> MGSSHHHHHHSSGENLYFQGHMSNTSWRKSEVLAVPLQPTLQQEVILARMEQILASRALTDDERAQLLYERGVLYDSLGLRALARNDFSQALAIRPDMPEVFNYLGIYLTQAGNFDAAYEAFDSVLELDPTYNYAHLNRGIALYYGGRDKLAQDDLLAFYQDDPNDPFRSLWLYLAEQKLDEKQAKEVLKQHFEKSDKEQWGWNIVEFYLGNISEQT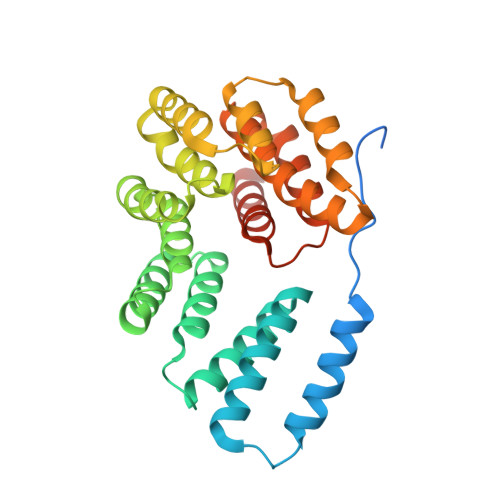LMERLKADATDNTSLAEHLSETNFYLGKYYLSLGDLDSATALFKLAVANNVHNFVEHRYALLELSLLGQDQDDLAESDQQ>MEDFKKIVNNIRLKDTFDFKLAAFPNQNYDQLLPSQIYKNYYQGIEIQQHKYQNELDIKIINFLYPDGDFGSANKNGTLKLSLMLTDKKNNQVYYKLLEVSGFKSNPYGVDENGTIPGLEHHHHHH[3x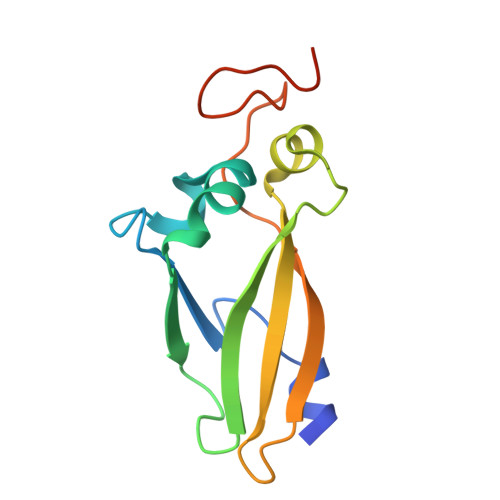]~{N}-[(2~{R},3~{R},4~{R},5~{S},6~{R})-5-[(2~{S},3~{R},4~{S},5~{S},6~{R})-4-[[1-[[3-[(~{Z})-3-[bis(azanyl)methylideneamino]prop-1-enyl]phenyl]methyl]-1,2,3-triazol-4-yl]methoxy]-6-(hydroxymethyl)-3,5-bis(oxidanyl)oxan-2-yl]oxy-6-(hydroxymethyl)-4-oxidanyl-2-prop-2-enoxy-oxan-3-yl]ethanamide 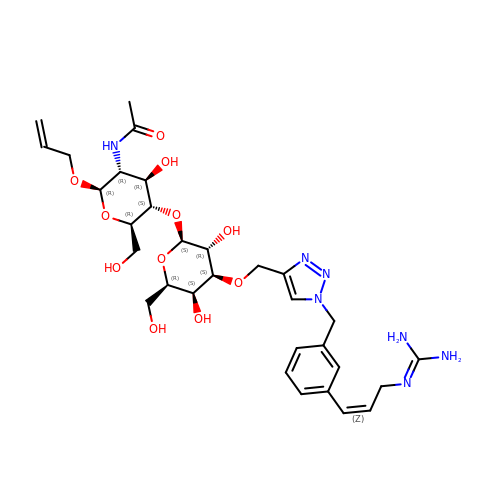| C31 H45 N7 O11 | WAFWFCVAGPTDEW-ORJNFUHYSA-N> TLSILVAHDLQRVIGFENQLPWHLPNDLKHVKKLSTGHTLVMGRKTFESIGKPLPNRRNVVLTSDTSFNVEGVDVIHSIEDIYQLPGHVFIFGGQTLFEEMIDKVDDMYITVIEGKFRGDTFFP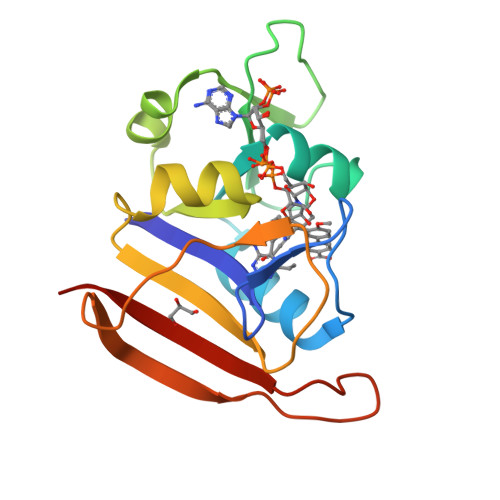PYTFEDWEVASSVEGKLDEKNTIPHTFLHLIRKLEH>[12x]MGLTVQKINWEQVKEWDRKYLMRTFSTQNEYQPVPIESTEGDYLITPGGTRLLDFFNQLCCVNLGQKNQKVNAAIKEALDRYGFVWDTYATDYKAKAAKIIIEDILGDEDWPGKVRFVSTGSEAVETALNIARLYTNRPLVVTREHDYHGWTGGAATVTRLRSFRSGLVGENSESFSAQIPGSSCSSAVLMAPSSNTFQD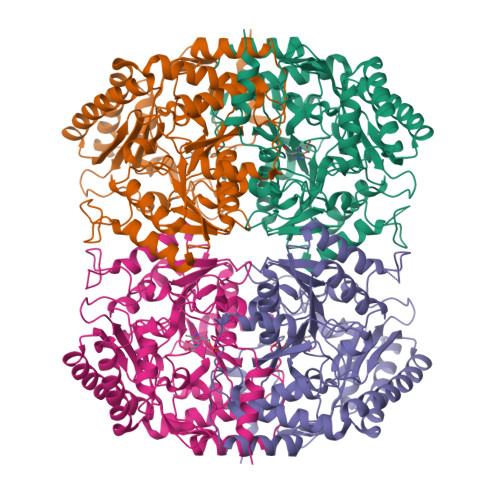SNGNYLKDENGELLSVKYTRRMIENYGPEQVAAVITEVSQGVGSTMPPYEYVPQIRKMTKELGVLWISDEVLTGFGRTGKWFGYQHYGVQPDIITMGKGLSSSSLPAGAVVVSKEIAAFMDKHRWESVSTYAGHPVAMAAVCANLEVMMEENLVEQAKNSGEYIRSKLELLQEKHKSIGNFDGYGLLWIVDIVNAKTKTPYVKLDRNFRHGMNPNQIPTQIIMEKALEKGVLIGGAMPNTMRIGASLNVSRGDIDKAMDALDYALDYLESGEWQQSALEHHHHHH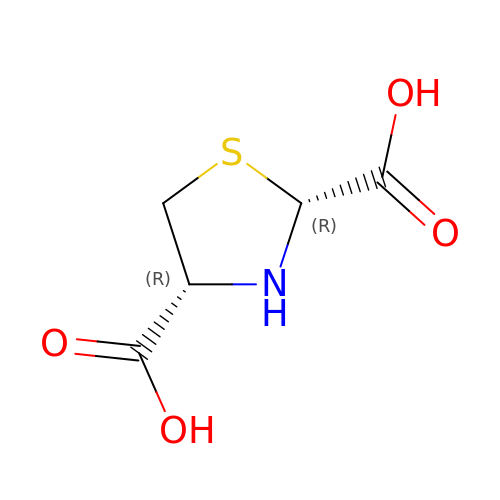(2~{R},4~{R})-1,3-thiazolidine-2,4-dicarboxylic acid | C5 H7 N O4 S | DAXBISKSIDBYEU-STHAYSLISA-N More recently, it was reported that a third protein SepCysE (SepRS/SepCysS pathway enhancer) is necessary for coupling the consecutive two reactions and for enhancing tRNACys binding. Thus, the SepRS, SepCysE, and SepCysS ternary complex (named the transsulfursome) is responsible for the whole process. In the present study, the structures of the binary complex of SepRS and SepCysE, and the ternary complex of SepCysE, SepCysS, and tRNACys from Methanocaldococcus jannaschii have been solved. On the basis of these results, we propose the scheme of the tRNA-dependent cysteine biosynthesis by the indirect pathway, where multidomain SepCysE binds SepRS and SepCysS to assemble into a functional unit (transsulfursome) and mediates the transfer of tRNA substrate between the active sites of SepRS and SepCysS via flexible linkers.

During the study of the quaternary complex SepRS-SepCysE-SepCysS-tRNACys, we serendipitously obtained the crystal of the ternary complex SepRS-SepCysE-SepCysS. In the electron density map, whole SepRS and the N-terminal helix (Met1–Lys24) of SepCysE(N-helix) were visible. However, the remaining components of SepCysE and SepCysS were disordered in the crystal, although there was enough space in the unit cell to accommodate the entire complex. SepRS was organized as a tetramer with 222 local symmetry (one of the two-fold axes is crystallographic), as previously observed. A pair of N-terminal helices (N-helices) of the dimeric SepCysE wound around each other to form a coiled-coil structure and were tightly bound to the SepRS with their two-fold axes aligned. Most of these residues (Leu9, Ile10, and Ile17) plus Ile14 were clustered with the hydrophobic residues in three pairs of loops ((loop 1: 376–380 ILDEF), (loop 2: 411–414 FNGE), and (loop 3: 494–498 ALVSN)) locating at the interface of two anticodon domains of the SepRS dimer and contributed to the formation of the complex together with some hydrogen bonds. Whereas deletion mutants of each of the three loops of SepRS showed no significant effect on binding, the double-loop deletion mutants did not bind SepCysE, suggesting these loops together contribute to the interaction with SepCysE. Likewise, N-helix deletion mutant SepCysE(ΔN-helix) completely lost the ability to bind SepRS. This structural and mutational evidence suggested that the SepCysE dimer tightly binds to the SepRS dimer by inserting its coiled-coil N-terminal helices into the interface of the SepRS dimer, which reinforces the stable architecture of transsulfursome. ATP was observed in the active sites of SepRS.

>[2x]MGSSMKLKHKRDDKMRFDIKKVLELAEKDFETAWRETRALIKDKHIDNKYPRLKPVYGKPHPVMETIERLRQAYLRMGFEEMINPVIVDEMEIYKQFGPEAMAVLDRCFYLAGLPRPDVGLGNEKVEIIKNLGIDIDEEKKERLREVLHLYKKGAIDGDDLVFEIAKALNVSNEMGLKVLETAFPEFKDLKPESTTLTLRSHMTSGWFITLSSLIKKRKLPLKLFSIDRCFRREQREDRSHLMSYHSASCVVVGEDVSVDDGKVVAEGLLAQFGFTKFKFKPDEKKSKYYTPETQTEVYAYHPKLGEWIEVATFGVYSPIALAKYNIDVPVMNLGLGVERLAMIIYGYEDVRAMVYPQFYEYRLSDRDIAGMIRVDKVPILDEFYNFANELIDICIANKDKESPCSVEVKREFNFNGERRVIKVEIFENEPNKKLLGPSVLNEVYVYDGNIYGIPPTFEGVKEQYIPILKKAKEEGVSTNIRYIDGIIYKLVAKIEEALVSNVDEFKFRVPIVRSLSDINLKIDELALKQIMGENKVIDVRGPVFLNAKVEIK;>MNHMRVEYSKDLIRKGISTISQLKKAKIRVEKDDKKISYKDAKPGKIDVNEFKKAIYLLIEADDFLYKKAPKHELNEEEAKEFCKLIIKCQEHLNKILANFGFEFEEKEIDEGALYIVSNKKLFKKLKNKNPNLKVVCTEGMLDIEDMRAIGVPEKALEGLKKKVEIARKNVERFIEKYKPEKIFVVVEDDKDELLYLRAKNLYNAEKLDADEILD[2x]> MKTSAKFLSFAVSFVLLIIASTSFAEGPVTATKPKEAGFTSEGLARIDAYLKNEIQAKTMPGAVMMIKRNGETAYFSSFGLRDPDTKEPMTAETIFRIYSMSKPITTVAAMMLVEEGKLQLDEPVSKYIPSFANVKVGVETKGENGMALETGPVKRAITIQDLMRHTSGITYGFVGDGLVKKAYIASNLFDGDFDNAEFAERIAKLPLVYQPGTTWDYGHSTDILGRVVEVVSGKSLYQFEKERLLDPLGMKDTGFYVTDPAKKSLVAEAMPNDRKIGGSEMFDPRVQKKWEPGGQGMVSTIGDYARFTQMVLNGGTLDGKRYLSPKTIAYMGSNHIPQA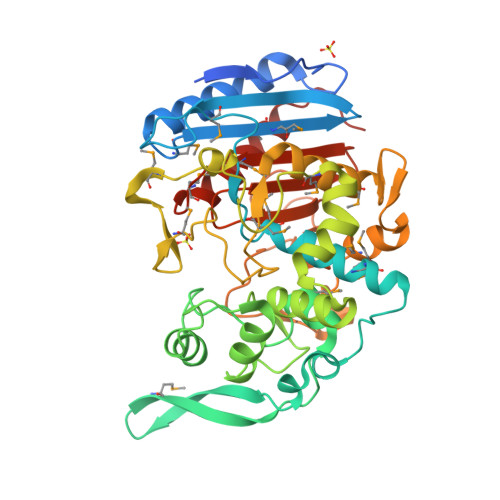SGIVPGAYYLPGPGVGFGLGFAVRTEAGVTPVEGSVGDLSWGGAGGTVFWIDPKENLTVVFMAPMVSPRARVWRTLRNIVYGAFDRLEHHHHHH>SNAMNAIIIDDHPLAIAAIRNLLIKNDIEILAELTEGGSAVQRVETLKPDIVIIDVDIPGVNGIQVLETLRKRQYSGIIIIVSAKNDHFYGKHCADAGAN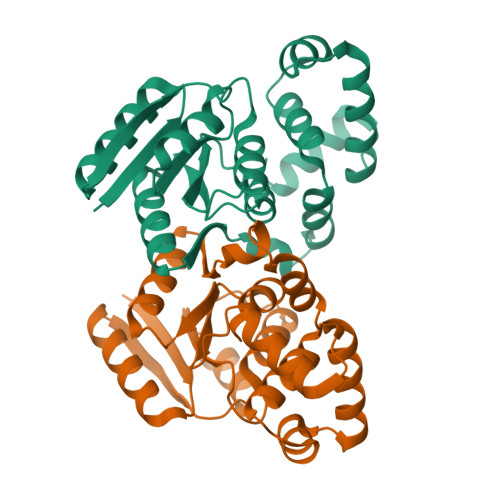GFVSKKEGMNNIIAAIEAAKNGYCYFPFSLNRFVGSLTSDQQKLDSLSKQEISVMRYILDGKDNNDIAEKMFISNKTVSTYKSRLMEKLECKSLMDLYTFAQRNKIG[4x]>MSLITVNTLQKMKAAGEKIAMLTAYESSFAALMDDAGVEMLLVGDSLGMAVQGRKSTLPVSLRDMCYHTECVARGAKNAMIVSDLPFGAYQQSKEQAFAAAAELMAAGAHMVKLEGGVWMAETTEFLQMRGIPVCAHIGLTPQSVFAFGGYKVQGRGGKAQALLNDAKAHDDAGAAVVLMECVLAELAKKVTETVSCPTIGIGAGADCDGQVLVMHDMLGIFPGKTAKFVKNFMQGHDSVQAAVRAYVAEVKAKT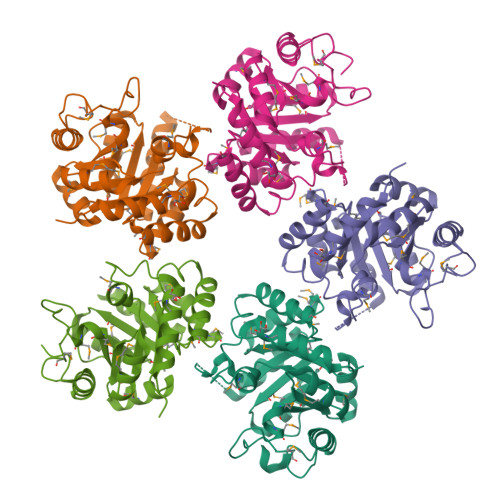FPAAEHIFADEGGSHHHHHH[5x]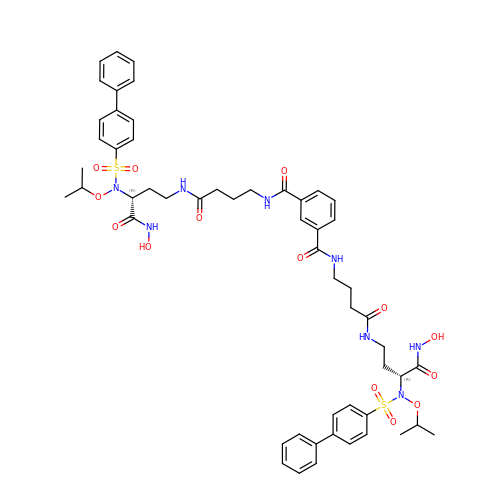N,N'-bis(4-{[(3R)-3-[(biphenyl-4-ylsulfonyl)(propan-2-yloxy)amino]-4-(hydroxyamino)-4-oxobutyl]amino}-4-oxobutyl)benzene-1,3-dicarboxamide | C54 H66 N8 O14 S2 | QTGQZAQZBAEHLR-URZIEALYSA-N>[2x]GP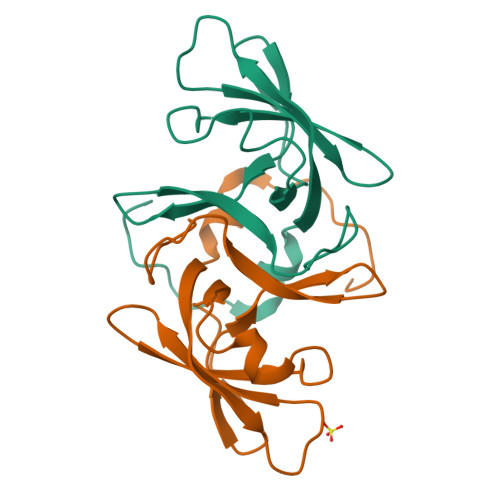MEEKALIGIEDFLKVDLRVAKVLSAERVEGSEKLLKLTLSLGDEERTVVAGIAKYYTPEELVGKKIVIVANLKPRKIFGIESQGMILAASDGENLSVIVPDRDVKEGAKLS>[2x]MQAVRLFQGYLW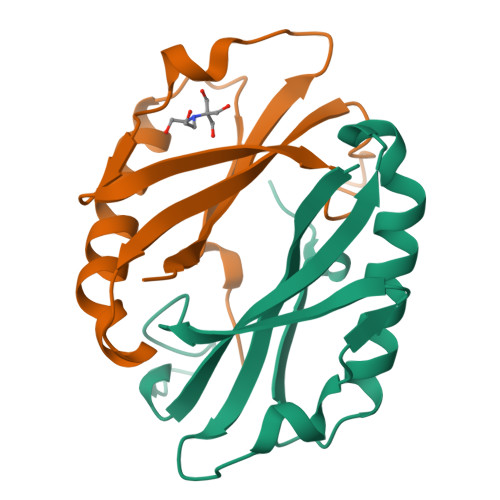HPRALALDLKALLPGEVAGARLLWDEVPPPTPFFEDGTPTHTQRFYQLTLLVLTEEPPEALKPLAEEAAEALGEVLEGLPPEVGWLLLEDLRPL> MNVNNPNQMTVTPVYNGCDSG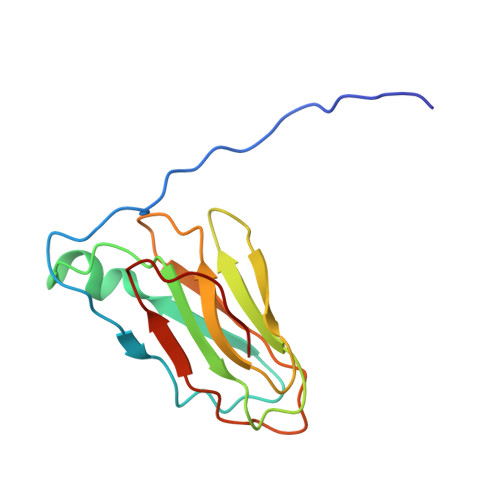EGPQSVRGYFDAVAGENVKYDLTYLADTQGFTGVQCIYIDNAENDGAFEIDVEETGQRIKCPAGKQGYFPLLVPGRAKFVARHLGSGKKSVPLFFLNFTIAQGVW>GHMWQENKSWNAHFTEHKSQGVVVLWNENKQQGFTNNLKRANQAFLPASTFKIPNSLIALDLGVVKDEHQVFKWDGQTRDIATWNRDHNLITAMKYSVVPVYQEFARQIGEARMSKMLHAFDYGNEDISGNVDSFWLDGGIRISATEQISFLRKLYHNKLHVSERSQRIVKQAMLTEANGDYIIRAKTGYSTRIEPKIGWWVGWVELDDNVWFFAMNMDMPTSDGLGLRQAITKEV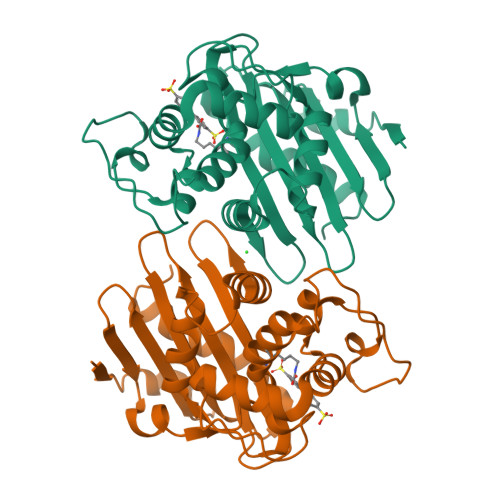LKQEKIIP[2x]> DVPVNLYRPNAPFIGKVISNEPLVKEGGIGIVQHIKFDL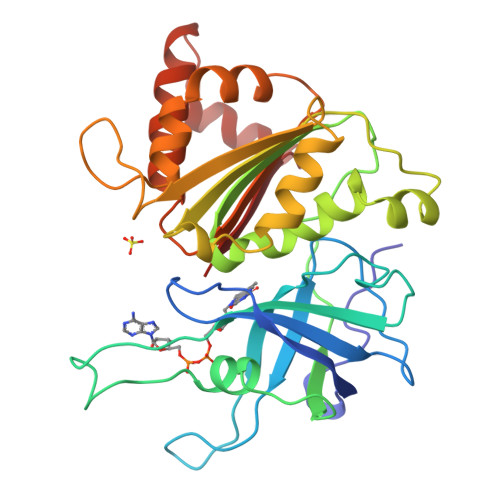TGGNLKYIEGQSIGIIPPGVDKNGKPEKLRDYSIASTRHGDDVDDKTISLCVRQLEYKHPESGETVYGVCSTYLTHIEPGSEVKITGPVGKEMLLPDDPEANVIMLATGTGIAPMRTYLWRMFKDAERAANPEYQFKGFSWLVFGVPTTPNILYKEELEEIQQKYPDNFRLTYAISREQKNPQGGRMYIQDRVAEHADQLWQLIKNQKTHTYICGLRGMEEGIDAALSAAAAKEGVTWSDYQKDLKKAGRWHVETY N5-(1-IMINO-3-BUTENYL)-L-ORNITHINE | C9 H20 N3 O2 | 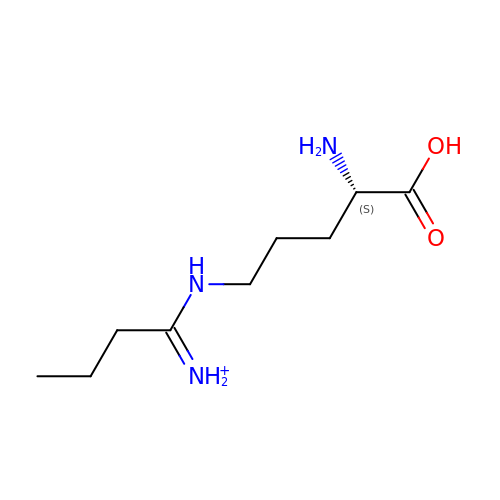KRILJVOCVSUPMA-ZETCQYMHSA-O>TMAASQTSQTVASHVPFADLCSTLERIQKSKGRAEKIRHFREFLDSWRKFHDALHKNHKDVTDSFYPAMRLILPQLERERMAYGIKETMLAKLYIELLNLPRDGKDALKLLNYRTPTGTHGDAGDFAMIAYFVLKPRCLQKGSLTIQQVNDLLDSIASNNSAKRKDLIKKSLLQLITQSSALEQKWLIRMIIKDLKLGVSQQTIFSVFHNDAAELHNVTTDLEKVCRQLHDPSVGLSDISITLFSAFKPMLAAIADIEHIEKDMKHQSFYIETKLDGERMQMHKDGDVYKYFSRNGYNYTDQFGASPTEGSLTPFIHNAFKADIQICILDGEMMAY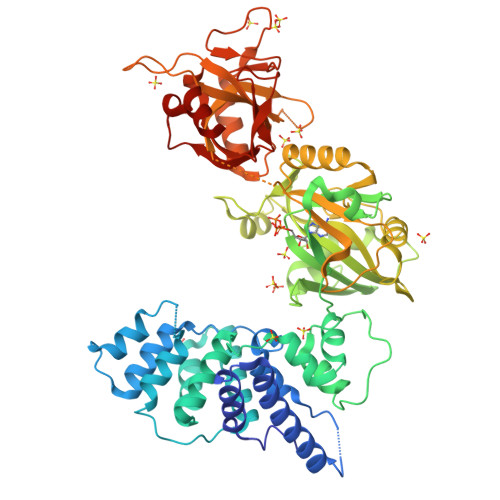NPNTQTFMQKGTKFDIKRMVEDSDLQTCYCVFDVLMVNNKKLGHETLRKRYEILSSIFTPIPGRIEIVQKTQAHTKNEVIDALNEAIDKREEGIMVKQPLSIYKPDKRGEGWLKIKPEYVSGLMDELDILIVGGYWGKGSRGGMMSHFLCAVAEKPPPGEKPSVFHTLSRVGSGCTMKELYDLGLKLAKYWKPFHRKAPPSSILCGTEKPEVYIEPCNSVIVQIKAAEIVPSDMYKTGCTLRFPRIEKIRDDKEWHECMTLDDLEQLRGKASGK[2x]> MRGSHHHHHHGSMPVAGSELPRRPLPPA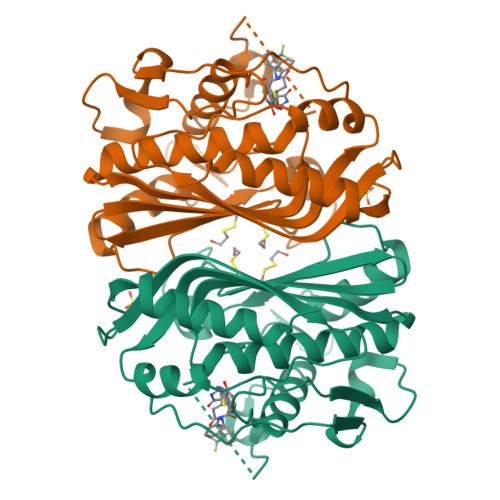AQERDAEPRPPHGELQYLGQIQHILRCGVRKDDRTGTGTLSVFGMQARYSLRDEFPLLTTKRVFWKGVLEELLWFIKGSTNAKELSSKGVKIWDANGSRDFLDSLGFSTREEGDLGPVYGFQWRHFGAEYRDMESDYSGQGVDQLQRVIDTIKTNPDDRRIIMCAWNPRDLPLMALPPCHALCQFYVVNSELSCQLYQRSGDMGLGVPFNIASYALLTYMIAHITGLKPGDFIHTLGDAHIYLNHIEPLKIQLQREPRPFPKLRILRKVEKIDDFKAEDFQIEGYNPHPTIKMEMAV>[2x]SGPRPRLWEGQDVLARWTDGLLYLGTIKKVDSAREVCLVQFEDDSQFLVLWKDISPAALPGEELLCCVCRSETVVPGNRLVSCEKCRHAYHQDCHVPRAPAPGEGEGASWVCRQCVFAIATKRGGALKKGPYARAMLGMKLSLPYGLKGLDWDAGHL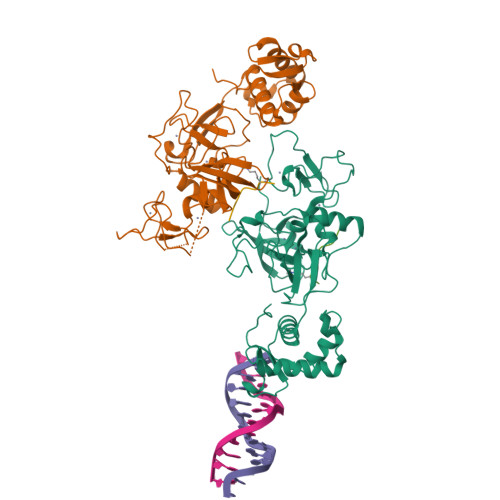SNRQQSYCYCGGPGEWNLKMLQCRSCLQWFHEACTQCLSKPLLYGDRFYEFECCVCRGGPEKVRRLQLRWVDVAHLVLYHLSVCCKKKYFDFDREILPFTSENWDSLLLGELSDTPKGERSSQLLSALNSHKDRFISGREIKKRKCLFGLHARTPPPVELLTGDGAPTSFPSGQGPGGG;>[2x]APATGGVKKPHRY> SRI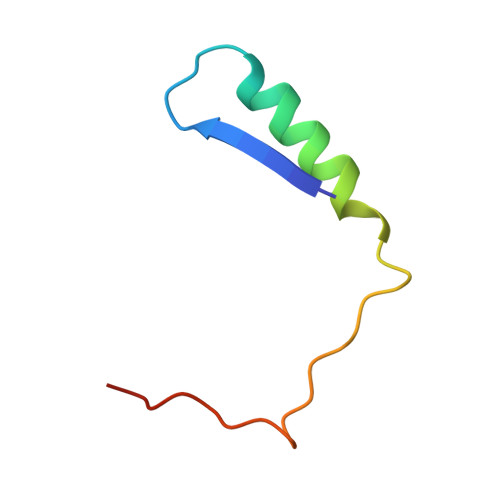LVSIGESFGTSEKFQKINQMVCNSDRVLKRSAEGSNPPKPLKK>GSRATVFKLGLFKSLFLCSFHDITRLFKNDKTTNQQWVLAVFGLAEVFFEASFELLKKQCSFLQMQKRSHEGGTCAVYLICFNTAKSRETVRNLMANMLNVREECLMLQPPKIRGLSAALFWFKSSLS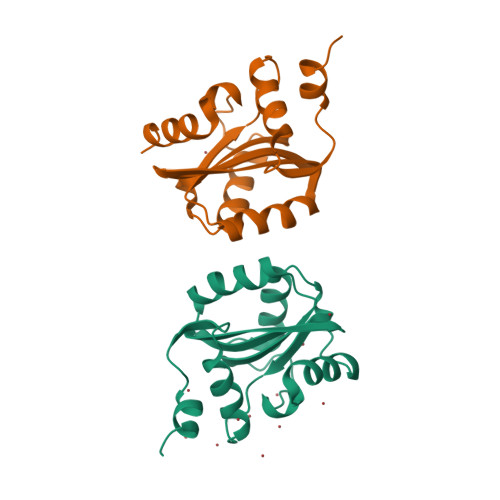PATLKHGALPEWIRAQTTLN[2x]>[2x]MGSSRTMTVDTGEELRAFVEGLVESGDYKTNSEVIRDGLRLLQEKTAGSKLAALRLEHHHHHH

Recently, PrpTA was found to be a pMBL6842-encoded type II TAS with the unique function to regulate the plasmid replication in Pseudoalteromonas rubra. It consists of stable PrpT toxin and labile PrpA antitoxin canonically positioned adjacently within the same operon. In this study, we reported for the first time the high-resolution structure of the PrpT:PrpA2:PrpT heterotetramer and two forms of crystal structures of truncated antitoxin-PrpA2–54. In addition, PrpA could also competitively bind to the iteron sequences in the ori, interfering with the binding of replication initiator RepB to the ori site, thus preventing the overreplication of the plasmid.

Considering the theoretical relative molecular weight of PrpT (∼11.4 kDa) and PrpA (∼11.66 kDa), our SEC-MALS results reflected that PrpTA complex, PrpAFL and PrpA2–54 present an estimated absolute mass matching tetramer, tetramer and dimer, respectively. Like other members from the RHH family, PrpA monomer polymerizes in solutions and crystals in a highly symmetrical manner via a local twofold axis to form a two-stranded antiparallel β-sheet. Moreover, the comparative structural analysis highlighted that PrpA2–54 dimers are similar to each other with an r.m.s.d. value of ∼1.38 Å over 96 residues. Thus, only the interface that existed in PrpA2–54-form II will be described in detail here. PISA analysis reflected that the hydrogen bond/salt bridge interaction network of dimerization interface is primarily offered by Met6, Val8, Asp9, Ser31, and Arg35 from each monomer together with Arg15A/B, Thr10A/B, Arg54A, Arg4B, and Asp26B for the PrpA2–54 (or symmetric Thr7A/B, Glu13A/B and asymmetric Ser3B for PrpAFL in PrpTA complex). The dimerization interface in PrpTA or PrpA2–54-form II buries roughly 1700 Å2 with the nearly identical negative ΔG value (∼24 kcal/mol) corresponding to hydrophobic interfaces. Except for the asymmetric Arg54A-ASP26B contact in PrpA2–54, the protein backbones of PrpA2–54 or PrpAFL project away from the dimer interface without further intra- or inter-contacts, suggesting the flexibility of PrpACTD. PrpA2–54-form I and II crystal structures both contain a doughnut-shaped hexadecamer formed by eight homodimers organized in a cogwheel-like form via inter-dimer interface dominated by salt bridges and hydrogen bonds. A circular hexadecamer (∼112.58 kDa) consisting of 8 PrpA2–54 dimers could be found in both forms of PrpA2–54 crystals. The maximum diameter of the annular doughnut-like hexadecamer is ∼80 Å and that of the hole in the center is approximately 22 Å.> MAEQTVEAPSVDARAWILMDYASGKVLAEGNADEKLDPASLTKIMTSYVVGQALKADKIKLTDMVTVGKDAWATGNPALRGSSVMFLKPGDQVSVADLNKGVIIQSGNDACIALADYVAGSQESFIGLMNGYAKKLGLTNTTFQTVHGLDA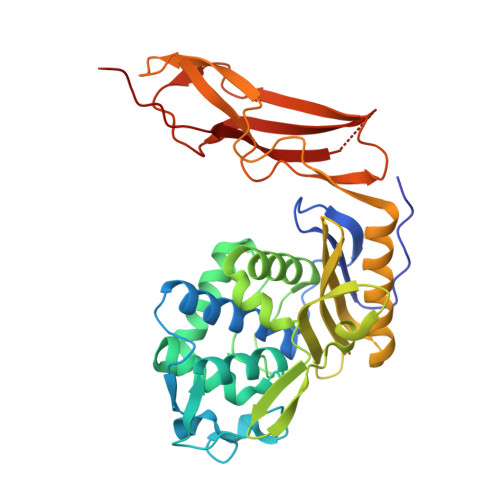PGQFSTARDMALLGKALIHDVPEEYAIHKEKEFTFNKIRQPNRNRLLWSSNLNVDGMKTGTTAGAGYNLVASATQGDMRLISVVLGAKTDRIRFNESEKLLTWGFRFFETVTPIKPDATFVTQRVWFGDKSEVNLGAGEAGSVTIPRGQLKNLKASYTLTEPQLTAPLKKGQVVGTIDFQLNGKSIEQRPLIVMENVEEGG>MKKGHHHHHHGAISLITALVRSHVDTTPDPSCLDYSHYEEQSMSEADKVQQFYQLLTSSVDVIKQFAEKIPGYFDLLPEDQELLFQSASLELFVLRLAYRARIDDTKLIFCNGTVLHRTQCLRSFGEWLNDIMEFSRSLHNLEIDISAFACLCALTLITERHGLREPKKVEQLQMKIIGSLRDHVTYNAEAQKK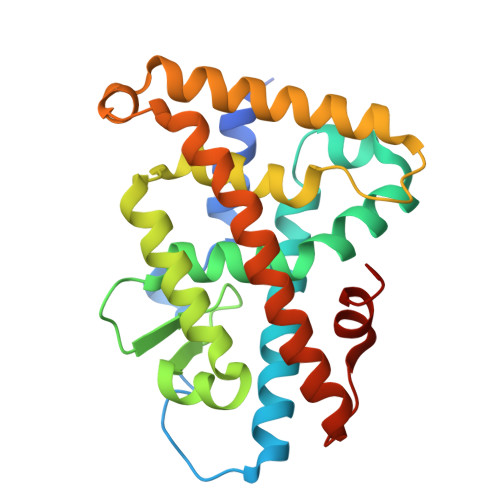QHYFSRLLGKLPELRSLSVQGLQRIFYLKLEDLVPAPALIENMFVTTLPF[2x]> IPIFLSVLQSIEPEVVYAGYDNTQPDT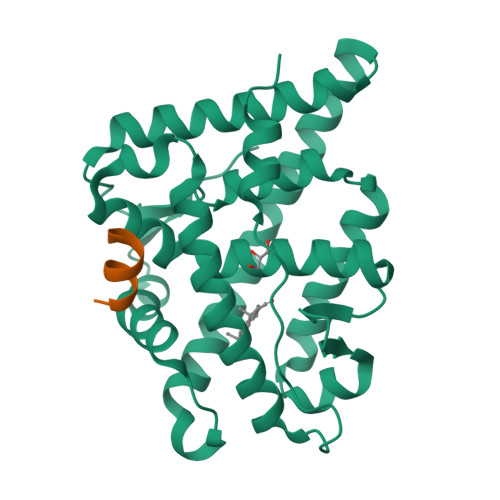SASLLTSLNELGERQLVRVVKWAKALPGFRNLHVDDQMTLIQYSWMGVMVFAMGWRSYKNVNSRMLYFAPDLVFNEQRMQKSTMYNLCVRMRHLSQEFVWLQVTQEEFLCMKALLLFSIIPVEGLKNQKYFDELRMNYIKELDRVISFQGKNPTSSSQRFYQLTKLLDSLQPIVRKLHQFTFDLFVQSQSLSVEFPEMMSEIISAQVPKILAGMVKPLLFH;> ALLRYLLDK>[4x]MQATVHESKQSIMQRILTVFVFTLLIATVGLFIGQFVPVALMLPLSILEVAMIILAFWMRRRKAVGYAFVYTFAFVSGITLFPIVSHYASIAGAYVVLEAFGSTFVIFAVLGTIG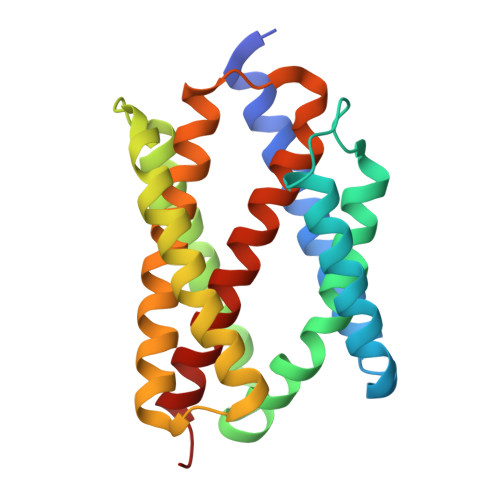AKMKKDLSFLWSFLLVAVLALAVVGIFNIFSPLNSAAMMAYSVIGTIVFSLYILYDLNQIKHRHITEDLIPVMALSLYLEFINLFINLLRFFGILSSDD>[2x]SSGSRD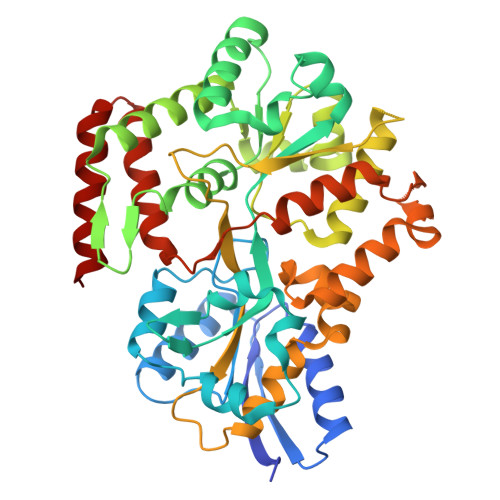DTQDVIGGKIVMYAAPGDNVQSEIRNIVRSKYPNVEFQVVSFNNADEFKSRLLTELMAGEGPDVIVLSPSTKKGSITIETMRKLVESGVFCDLEPYISKDESINLSEYNETVLNSGVINGKRYFIPIAYDVPIFWTANSILEENNIKDEIANWTLKDMADFAVQFKEKNSDNYLFGYGDGFIRNIMYANWREFVDYENKQASFDSQEFVEFLEAIGAIEKAGICDEKLIKEYTGMEFEALKHGKITLISSTEYPINPWELWYRNSHINYYFNPDSIRLSKFPTFGDLGRIVAHPTDIVAINKNSKNKATAYEVLKVFLSKEIQSSQQFRDRMGIPVNDEAIRELIEKYSGEEGKTTLPVGMTINETMDTVPLPESVVAEYNSIINGVTECVLVDEQIIDFMIEGFNEYKNGKMSAKDAARMVQQKVNLFLNE> GSMSTINFANREINFKIVYYGPGLSGKTTNLKWIYSKVPEGRKGEMVSLATEDERTLFFDFLPLDIGEVKGFKTRFHLYTVPGQVFYNASRKLILRGVDGIVFVADSAPNRLRANAESMRNMRENLAEYGLTLDDVPIVIQVNKRDLPDALPVEMVRAVVDPEGKFPVLEAVATEGKGVFETLKEVSRLVLARVAGGS;>GSLVLYGAPYAAAVEVLEETLRETGARYALLIDRKGFVLAHKEALWAPKPPPLDTLATLVASNAAATQALAKLLGEARFQEEVHQGERMGLYVDEAGEHALLVLVFDETAPLGKVKLHGKAAAAALAAIAEEAL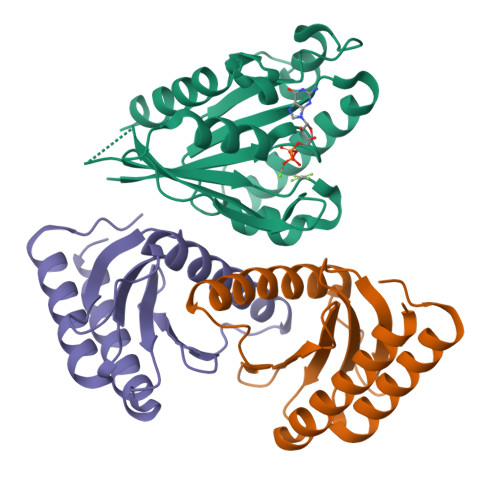AN[2x]> MTIDEIIEAIEKL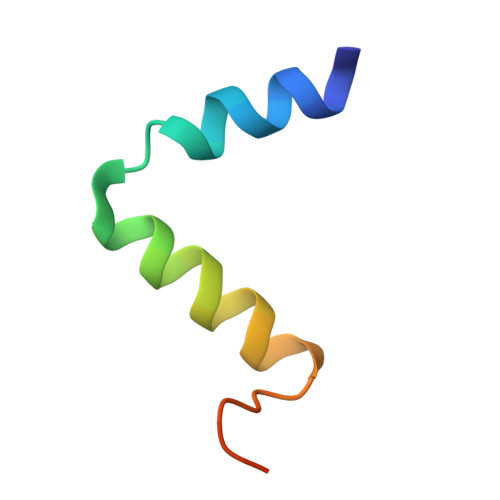TVSELAELVKKLEDKFGVTAAAPVAVA>MANVPGQKVGTDQGKGKSGSDALALFLKVFAGEVLTAFTRRSVTADKHIVRTIQNGKSAQFPVMGRTSGVYLAPGERLSDKRKGIKHTEKNITIDGLLTADVMIFDIEDAMNHYDVAGEYSNQLGEALAIAADGAVLAEMAILCNLPAASNENIAGLGTASVLEVGKKADLNTPAKLGEAIIGQLTIARAKLTSNYVPAGDRYFYTTPDNYSAILAALMPNAANYAALIDPETGNIRNVMGFVVVEVPHLVQGGAGGTRGADGISIASGQKHAFPATAAGAVKVAMDNVVGLFSHRSAVGTVKLRDLALERDRDVDAQGDLIVGKYAM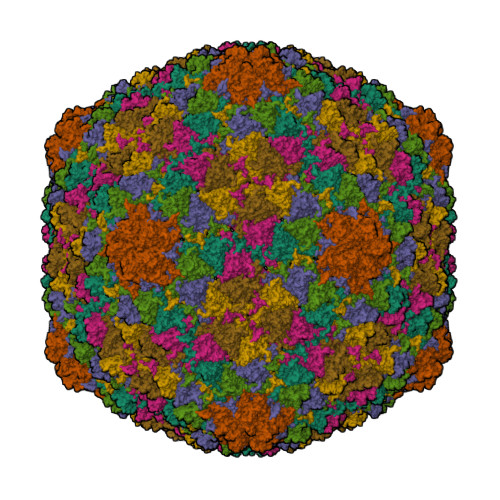GHGGLRPEAAGALVFSPAA[7x]> DEPGVATGNGQPVTGNWLAGASQGDGVPIPSQIADQLRGKEFKSWRDFREQFWVAVANDPELVKYFRKTNAKGMRDG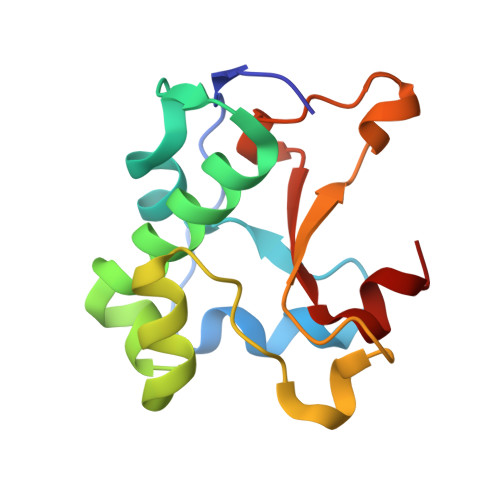LSPFTPKAEQAGGRDKYAIHHVVQISQGGAVYDIDNLRVMTPKMHIQV> EPLDESSVKKMILTFEKRSYKNQELRIKFPDNPEKFMESELDLNDIIQEMHVVATMPDLYHLLVELNAVQSLLGLLGHDNTDVSIAVVDLLQELTDIDTLHESEEGAEVLIDALVDGQVVALLVQNLERLDESVKEEADGVHNTLAIVENMAEFRPEMCTEGAQQGLLQWLLKRLKAKMPFDANKLYCSEVLAILLQDNDENRELLGELDGIDVLLQQLSVFKRHNPSTAEEQEMMENLFDSLCSCLMLSSNRERFLKGEGLQLMNLMLREKKISRSSALKVLDHAMIGPEGTDNCHKFVDILGLRTIFPLFMKSPRKIKKVGTTEKEHEEHVCSILASLLRNLRGQQRTRLLNKFTENDSEKVDRLM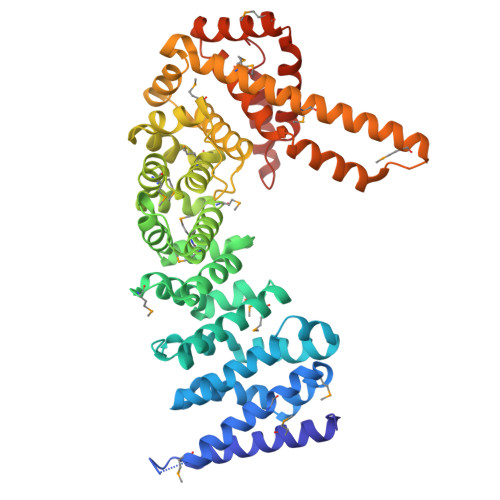ELHFKYLGAMQVADKKIEGEKHDMVRRGEIIDNDTEEEFYLRRLDAGLFVLQHICYIMAEICNANVPQIRQRVHQILNMRGSSIKIVRHIIKEYAENIGDGRSPEFRENEQKRILGLLENF>GGGRMEGESTLGVLSGFVLGALTFHHLNTDSDTEGFLLGEMKGEAKNSITDSQMDNVKVVYTIDIQKYIPCYRLFSFYNSLGEVNEHALKKVLSNVRKTVVGWYKFRRHSDQIMTFREQLLHRNLQTHLSSPELVFLLLTPSITTESCSTHCLEHALYKPQRGLFHRVPLVVTNLGMSDQLGYKTEPASCTSTVFSRAVRTHSSQFFNEDGSLKEVHKINEMYAAVQEELKSICQKVEQSEREVEKLLMDVNQLKEVRRTQQARATGAGEKNVQRNPQENILLCQALRTFFPESEVLHSCVISLKNRHISPSGCNVNHHVDVVDQLTLMVEYVYSPEASPVPTAQLRKRKALDTHDQGSVKRPRLLETESRPSVAASRSRHQDKASSSSLDIDIEMGSPEDDADYPRSPTF[2x];>GGGRMAVQVVQAVQAVHLESDAFLVCLNHALSTEKEEVMGLCIGELNDDIRSDSKFTYTGTEMRTVQEKMDTIRIVHIHSVIILRRSDKRKDRVEISPEQLSAASTEAERLAELTGRPMRVVGWYHSHPHITVWPSHVDVRTQAMYQMMDQGFVGLIFSCFIEDKNTKTGRVLYTCFQSIQAQKSSEYERIEIPIHIVPHITIGKVCLESAVELPKILCQEEQDAYRRIHSLTHLDSVTKIHNGSVFTKNLCSQMSAVSGPLLQWLEDRLEQNQQHLQELQQEKEELMEELSSLE[2x];>GGGRMSPEIALNRISPMLSPFISSVVRNGKVGLDATNCLRITDLKSGCTSLTPGPNCDRFKLHIPYAGETLKWDIIFNAQYPELPPDFIFGEDAEFLPDPSALHNLASWNPSNPECLLLVVKELVQQYHQFQCGRLRESSRLMFEYQTLLEEPQYGENMEIYAGKKNNWTGEFSARFLLKLPVDFSNIPTYLLKDVNEDPGEDVALLSVSFEDTEATQVYPKLYLSPRIEHALGGSSALHIPAFPGGGCLIDYVPQVCHLLTNKVQYVIQGYHKRREYIAAFLSHFGTGVVEYDAEGFTKLTLLLMWKDFCFLVHIDLPLFFPRDQPTLTFQSVYHFTNSGQLYSQAQK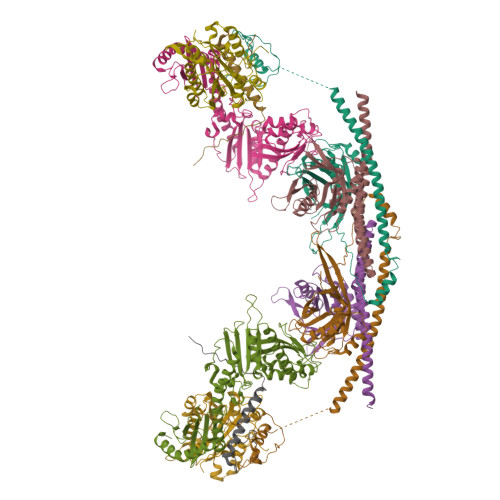NYPYSPRWDGNEMAKRAKAYFKTFVPQFQEAAFANGKL[2x];>GGGRMEVAEANSPTEEEEEEEEEGEETISEPRPHTRSNPEGAEDRALGAQASVGSRSEGEGEAATADGGAASVPGAGPKPWQVPASASEVQIRTPRVNCPEKVIICLDLSEEMSVPKLESFNGSRTNALNVSQKMVEMFVRTKHKIDKSHEFALVVVNDDSAWLSGLTSDPRELCSCLYDLETASCSTFNLEGLFSLIQQKTELPVTENVQTIPPPYVVRTILVYSRPPCQPQFSLTEPMKKMFQCPYFFFDIVYIHNGTEEKEEDMSWKDMFAFMGSLDTKGASYKYEVALAGPALELHNCMAKLLAHPLQRPCQTHASYSLLEEDEEAGEEEATV[2x];>[2x]GGGRHYYWGIPFCPAGVDPNQYTNVILCQLEVYQKSLKMAQRQLVKKRGFGEPVLPRPPFLIQN> MFVARSIAADHKDLIHDVSFDFHGRRMATCSSDQSVKVWDKSESGDWHCTASWKTHSGSVWRVTWAHPEFGQVLASCSFDRTAAVWEEIVGESNDKLRGQSHWVKRTTLVDSRTSVTDVKFAPKHMGLMLATCSADGIVRIYEAPDVMNLSQWSLQHEISCKLSCSCISWNPSSSRAHSPMIAVGSDDSSPNAMAKVQIFEYNENTRKYAKAETLMTVTDPVHDIAFAPNLGRSFHILAIATKDVRI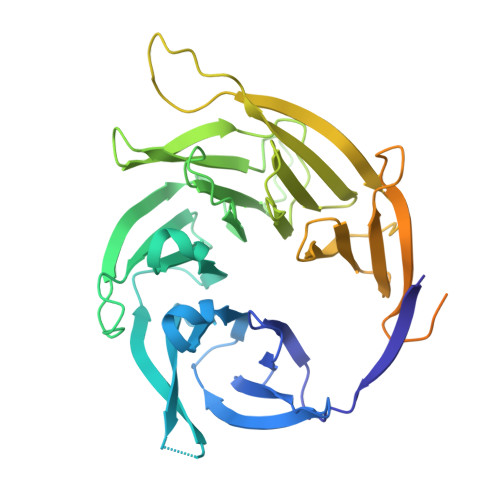FTLKPVRKELTSSGGPTKFEIHIVAQFDNHNSQVWRVSWNITGTVLASSGDDGCVRLWKANYMDNWKCTGILKGNGSPVNGSSQQGTSNPSLGSTIPSLQNSLNGSSAGRYFFTPLDSPRAGSRWSSYAQLLPPPPPPLVEHSCDADTANLQYPHPRRRYLSRPLNPLPENEGI>APECGERASGKRCPNGKCCSQWGYCGTTDNYCGQG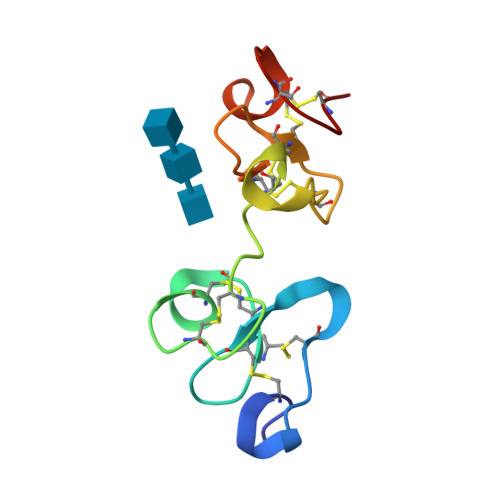CQSQCDYWRCGRDFGGRLCEEDMCCSKYGWCGYSDDHCEDGCQSQCD[2x]>[8x]MNKEDLLKKAFEAMENAYAPYSNYHVGACALMKDGTTFLGANIENASYGATNCGERSAIFAAYSNGYRADD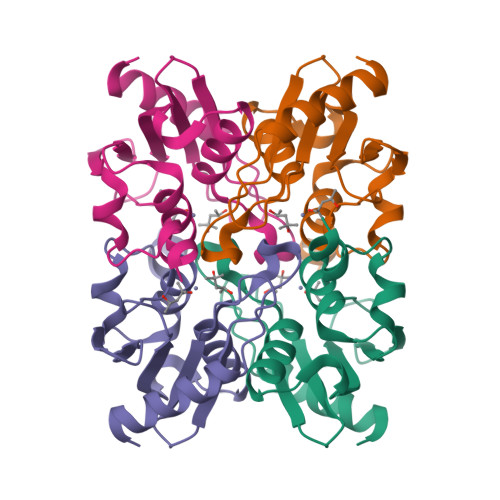IEALAIVTDGDRVGAPCGICRQVLSELLNDNTPIYLSNGKETLEKTIDELLPMRFTKEDLLGHHHHHHG>MAHHHHHHMGKPDPILGLGQDFRMDPAKRKVNLSIGVYRDDADQP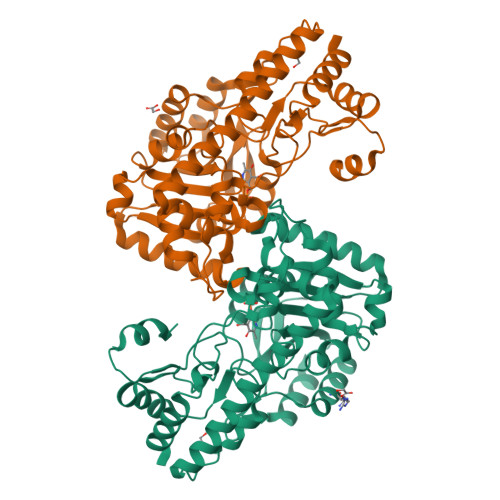FVLECVKQATLGTNMDYAPVTGIASFVEEAQKLCFGPTCAALRDGRIASCQTLGGTGALRIGGDLLNRFVANCNRIYGPDVGYPNHESIFAKAGMELTPYSYYDPATKGLNLAGMLECLDKAPEGSVILVHACAHNPTGVDPTHDDWRQVCDVIKRRNHIPFVDMAYQGFATGQLDYDAFVPRHLVDMVPNLIVAQSFSANFGLYGHRCGALHISTASAEEAKRLVSQLALLIRPMYSNPPLYGAWVVSSILKDPQLTALWKKELKQMSSRIAEVRKRLVSELKACGSVHDWSHIERQVGMMAYTGLTREQVELLRSEYHIYMTLNGRAAVSGLNSTNVEYVSQAIHNVTK[2x]> MSYTIESARNIFSSTQVADAVPATTAMFAKLNVDDQLAFLWYAYAELGRTITPAAPGKANLQLMEGIFNDIKQMSHEQQTQLMRDLASNADTPISRSYAYFGVNAKLGFWWQLGEWMKQGIVAPMPAGYQMSTQVKAVLEAVQRIDQSQQITVLRNTVVNMGFDPSLADKQQAEVINFKFPRASLSPQFTIEGVTEPTVLKYIEAMNADNFEAAVALFANNGALQPPFQKPIVGREA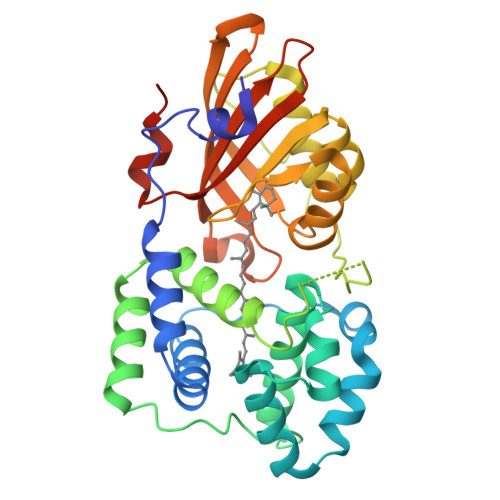ITAYLRDEGQGLVMKPTKGVSETIEDGYTQHKVTGTVETPWFGGNVGMNIAWRFLLDPQGQIYFVAIDLLASPKELLNLTRKHHHHHH>[2x]MNTNKNDTAFTVDLTNCDKEPIHIPGFVQPHGVLLAIKEPELTILQVSNNTYNCLGFHPEELLNQPLRKLLESEQIDFLNDCLTQEDIQIVNPVEFTIKTFQEPIIFDGIIHRSNGVVILELEPAILEKNNNYFRFYHLVKLAIGKLQSTKTVTEISQ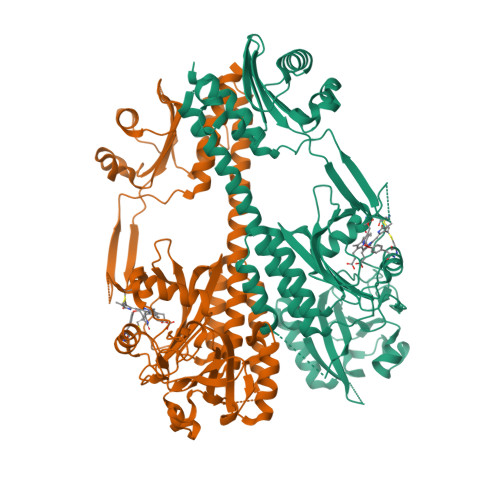IIVTEVRRITGFDRVMFYRFDRDWNGIVIAEDKQEHLPSYLDLHYPASDIPTPARKLYSQNWLRLIPDADYQAAAIVPTNNPLTDEPLDLSGSVLRSVSPCHIEYLHNMGVKASMSISIIKNNKLWGLIACHHQTPKYVPYEIRHACEFLGQVTSLEIATKEDNEDSESKIEIKSVLAKLVEYMSAEKSFIDGLINKQPNILNLVNAQGAAICFNKELYLLGNTPEKQDIQNLLLWIHNNIDEDIFYTDSLSQVYPEAEKFKDVASGLIALSISKTQNKYVLWFRPEEVQTVNWGGNPNQPVEVSENGGLHLSPRKSFELWKEIVRLKSLPWKSYEVNAAAELRGAIITVVLRKIDEHHHHHH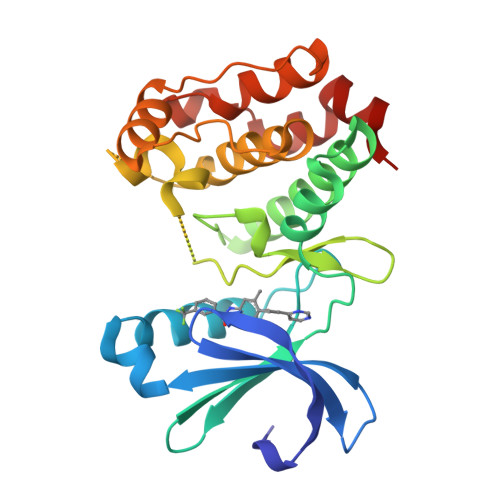>[2x]KRQWALEDFEIGRPLGKGKFGNVYLAREKQSKFILALKVLFKAQLEKAGVEHQLRREVEIQSHLRHPNILRLYGYFHDATRVYLILEYAPLGTVYRELQKLSKFDEQRTATYITELANALSYCHSKRVIHRDIKPENLLLGSAGELKIADFGWSVHAPSSRRTTLCGTLDYLPPEMIEGRMHDEKVDLWSLGVLCYEFLVGKPPFEANTYQETYKRISRVEFTFPDFVTEGARDLISRLLKHNPSQRPMLREVLEHPWITANSSKPS> ATRRYYLGAVELSWDYMQSDLGELPVDARFPPRVPKSFPFNTSVVYKKTLFVEFTDHLFNIAKPRPPWMGLLGPTIQAEVYDTVVITLKNMASHPVSLHAVGVSYWKASEGAEYDDQTSQREKEDDKVFPG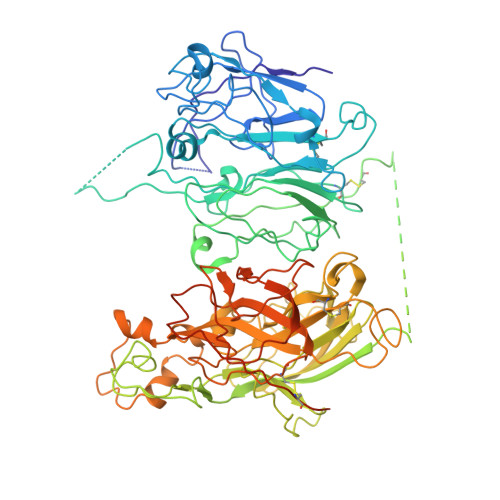GSHTYVWQVLKENGPMASDPLCLTYSYLSHVDLVKDLNSGLIGALLVCREGSLAKEKTQTLHKFILLFAVFDEGKSWHSETKNSLMQDRDAASARAWPKMHTVNGYVNRSLPGLIGCHRKSVYWHVIGMGTTPEVHSIFLEGHTFLVRNHRQASLEISPITFLTAQTLLMDLGQFLLFCHISSHQHDGMEAYVKVDSCPEEPQLRMKNNEEAEDYDDDLTDSEMDVVRFDDDNSPSFIQIRSVAKKHPKTWVHYIAAEEEDWDYAPLVLAPDDRSYKSQYLNNGPQRIGRKYKKVRFMAYTDETFKTREAIQHESGILGPLLYGEVGDTLLIIFKNQASRPYNIYPHGITDVRPLYSRRLPKGVKHLKDFPILPGEIFKYKWTVTVEDGPTKSDPRCLTRYYSSFVNMERDLASGLIGPLLICYKESVDQRGNQIMSDKRNVILFSVFDENRSWYLTENIQRFLPNPAGVQLEDPEFQASNIMHSINGYVFDSLQLSVCLHEVAYWYILSIGAQTDFLSVFFSGYTFKHKMVYEDTLTLFPFSGETVFMSMENPGLWILGCHNSDFRNRGMTALLKVSSCDKNTGDYYEDSYEDISAYLLSKNNAIEPRSFSQNPPVLKRHQR>MEMFQGLLLWLLLGVAGVWASRGPLRPLCQPINATLAAEKEACPVCITFTTSICAGYCPSMKRVLPVILPPMPQRVCTYHELRFASVRLPGCPPGVDPMVSFPVALSCHCGPCRLSSTDCGGPRTQPLACDHPPLPDI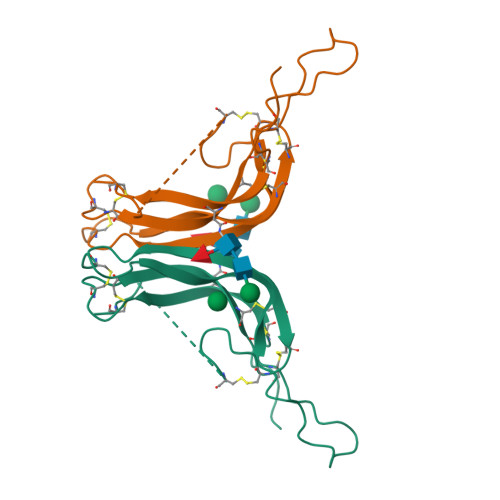LFL[2x]(2~{S})-~{N}1-(1-aminocarbonylindol-3-yl)-~{N}2-[3-(trifluoromethyloxy)phenyl]pyrrolidine-1,2-dicarboxamide 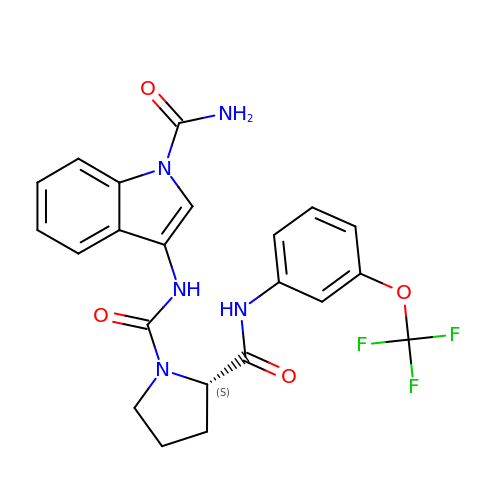| C22 H20 F3 N5 O4 | GPEWMCZCFCZAEI-SFHVURJKSA-N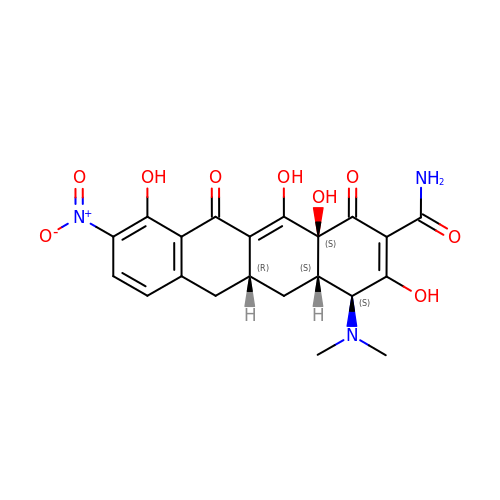(4S,4aS,5aR,12aS)-4-(dimethylamino)-3,10,12,12a-tetrahydroxy-9-nitro-1,11-dioxo-1,4,4a,5,5a,6,11,12a-octahydrotetracene-2-carboxamide | C21 H21 N3 O9 | IEJWCNPEOOQYLP-CROFIWJMSA-N> SLGGQIVLGGSDPQHYEGNFHYINLIKTGVWQIQMKGVSVGSSTLLCEDGCLALVDTGASYISGSTSSIEKLMEALGAKKRLFDYVVKCNEGPTLPDISFHLGGKEYTLTSADYVFQESYSSKKLCTLAIHAMDIPPPTGPTWALGATFIRKFYTEFDR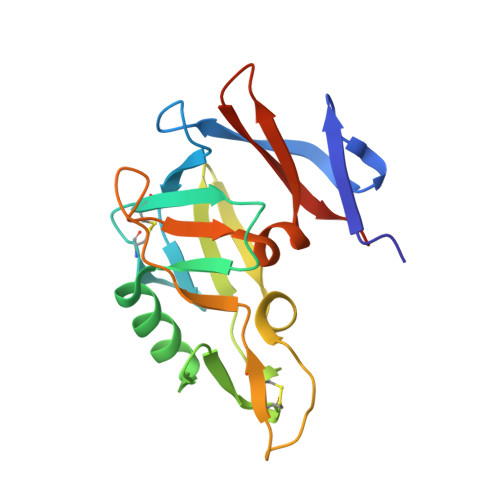RNNRIGFALARHHHHHH>MSKTQEFRPLTLPPKLSLSDFNEFIQDIIRIVGSENVEVISSKDQIVDGSYMKPTHTHDPHHVMDQDYFLASAIVAPRNVADVQSIVGLANKFSFPLWPISIGRNSGYGGAAPRVSGSVVLDMGKNMNRVLEVNVEGAYCVVEP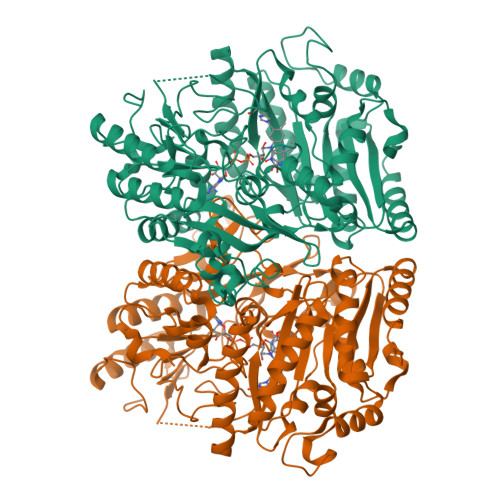GVTYHDLHNYLEANNLRDKLWLDVPDLGGGSVLGNAVERGVGYTPYGDHWMMHSGMEVVLANGELLRTGMGALPDPKRPETMGLKPEDQPWSKIAHLFPYGFGPYIDGLFSQSNMGIVTKIGIWLMPNPRGYQSYLITLPKDGDLKQAVDIIRPLRLGMALQNVPTIRHILLDAAVLGDKRSYSSRTEPLSDEELDKIAKQLNLGRWNFYGALYGPEPIRRVLWETIKDAFSAIPGVKFYFPEDTPENSVLRVRDKTMQGIPTYDELKWIDWLPNGAHLFFSPIAKVSGEDAMMQYAVTKKRCQEAGLDYIGTFTVGMREMHHIVCIVFNKKDLIQKRKVQWLMRTLIDDCAANGWGEYRTHLAFMDQIMETYNWNNSSFLRFNEVLKNAVDPNGIIAPGKSGVWPSQYSHVTWKL[2x]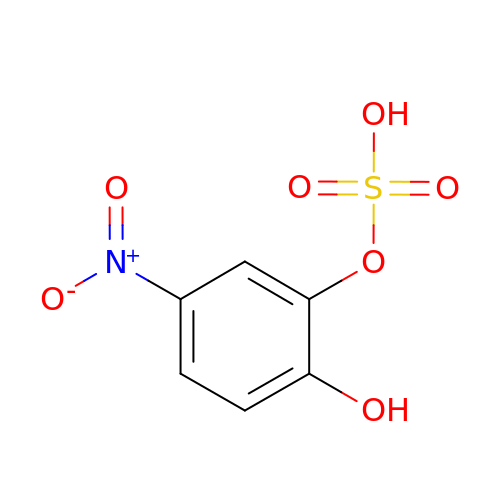N,4-DIHYDROXY-N-OXO-3-(SULFOOXY)BENZENAMINIUM | C6 H5 N O7 S | XMCCOOONGGUOLA-UHFFFAOYSA-N>MWSHPAVRKSSSKTIRSRSIWDDAHAMLEKAKAEGISTVWDRAAEQTPACKFCELGTTCRNCIMGPCRIANRKDGKMRLGVCGADADVIVARNFGRFIAGGAAGHSDHGRDLIETLEAVAEGKAPGYTIRDVAKLRRIAAELGVADAATRPAHDVAADLVTICYNDFGSRRNALAFLARAPQVRRDLWQRLGMTPRGVDREIAEMMHRTHMGCDNDHTSLLVHAARTALADGWGGSMIGTELSDILFGTPRPRQSTVNLGVLRKDAVNILVHGHNPVVSEMILAATREPAVRQAAQDAGAADINVAGLCCTGNELLMRQGIPMAGNHLMTELAIVTGAADAIVADYQCIMPSLVQIAACYHTRFVTTSPKGRFTGATHVEVHPHNAQERCREIVMLAIDAYTRRDPARVDIPSQPVSIMSGFSNEAILEALGGTPKPLIDAVVAGQIRGFVGIVGCNNPKIRQDSANVTLTRELIRRDIMVLATGCVTTAAGKAGLLVPEAASKAGEGLAAVCRSLGVPPVLHMGSCVDNSRILQLCALLATTLGVDISDLPVGASSPEWYSEKAAAIAMYAVASGIPTHLGLPPNILGSENVTAMALHGLQDVVGAAFMVEPDPVKAADMLEAHIVARRARLGLTS[2x]

The anaerobic, Ni-dependent CODH has a homodimeric structure containing a total of five metalloclusters, called the B-, C-, and D-clusters. The C-cluster is the site of CO/CO2 interconversion and is composed of a [Ni-3Fe-4S] cubane connected through a linking sulfide (SL) to a unique iron site (Feu). Here, we report the crystal structure of the CODH from Desulfovibrio vulgaris (DvCODH), which reveals a surprising and unprecedented conformational rearrangement of metal ions in the C-cluster and provides the first visualization of the cluster in an oxidized state. The overall fold and cluster placement of DvCODH is highly similar to other structurally characterized CODHs.

In the present work, we determined two structures of as-isolated DvCODH using two independent protein batches and much to our surprise, we observe different conformations of the C-cluster in each structure. A 2.50 Å resolution structure of as-isolated DvCODH (determined using protein batch 1) displays the canonical [Ni-3Fe-4S]-Feu C-cluster; the [Ni-3Fe-5S]-Feu state that was observed in structures of Carboxydothermus hydrogenoformans CODH-II is no longer thought to be catalytically relevant. The ligation of the C-cluster is conserved in DvCODH with four cysteines ligating the cubane portion of the cluster (Cys519 is the Ni ligand); one histidine (His266) and one cysteine (Cys302) ligate Feu. One noteworthy difference with respect to other CODHs is the identity of the D-cluster, a solvent-exposed Fe-S cluster at the dimer interface that serves as an electron conduit to the surface of the protein. Instead of the expected [4Fe-4S] cluster, the electron density is consistent with a [2Fe-2S] cluster as is the placement of cysteine residues in the primary structure. CODH sequence alignments reveal that instead of a C-X7-C D-cluster binding motif, DvCODH, as well as several uncharacterized CODHs, have a C-X2-C motif. This shortened C-X2-C motif appears to constrain the geometry of the ligating cysteine residues such that coordination to a [4Fe-4S] cluster is not possible.> GAMDPEFALSNEKKAKKVRFYRNGDRYFKGIVYAVSSDRFRSFDALLADLTRSLSDNINLPQ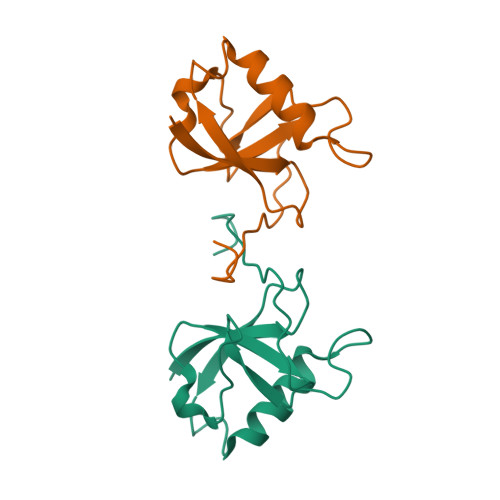GVRYIYTIDGSRKIGSMDELEEGESYVCSSDNFFDDVEYTKNVNPNWSVNV> MASAATGVRAVPGNENSLEIEELARFAVDEHNKKENALLEFVRVVKAKEQVDLTRFPVTTMYYLTLEAKDGGKKKLYEAKVWVKGYLLEELKHNFKELQEFKPVGDAAAAHHHH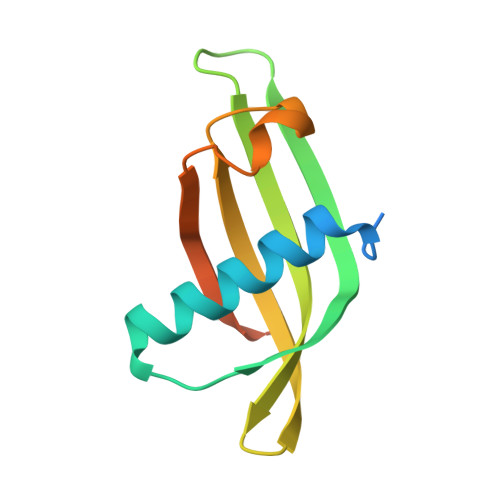HHHH> GLRQAVMLPEGEDLNEWIAVNTVDFFNQINMLYGTITEFCTEASCPVMSAGPRYEYHWADGTNIKKPIKCSAPKYIDYLMTWVQDQLDD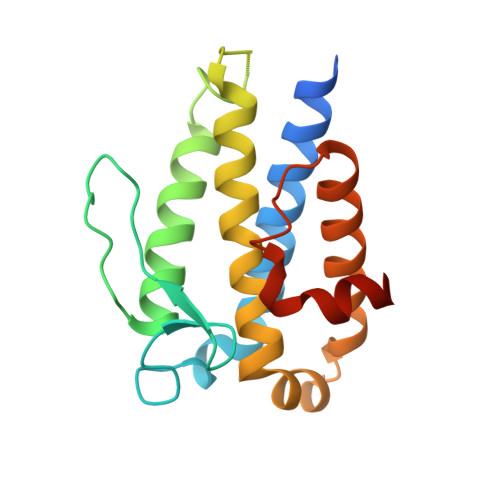ETLFPSKIGVPFPKNFMSVAKTILKRLFRVYAHIYHQHFDSVMQLQEEAHLNTSFKHFIFFVQEFNLIDRRELAPLQELIEKLGSKDR>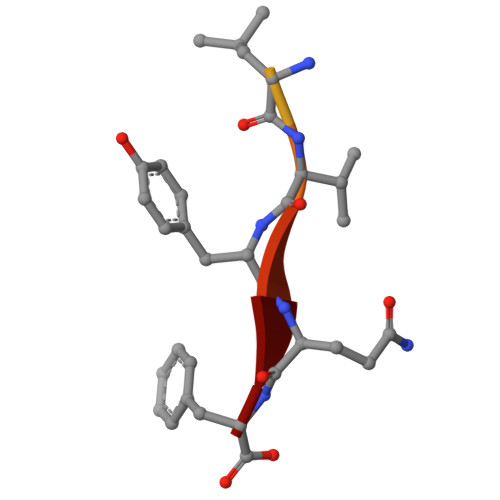 DNRLGLVYQF> MRGSHHHHHHGSMVAPTSNPGVPDELDGVPAVVDCDVHAVLPSPHSLIPYLDEYWADQLVAQLAPTYEPNYHPRGSAIAQHSDASVDENGRAATTAENLVKDVFADGFTDFAVVNCLYGVQQIHQPRREMAHARALNHWIANEWLDKDDRLRASIVVPQGSPRAAAEEIDFWSGDKRFVQVLLLGQSELLYGREINWPIWEAAEAAGLPVTLHIGGVFRQAPTSVGWPASHLEWYVGQQSNIEAQLNSIISEGILQKFPKTKILLSELGFNWLPPFMWKFDKLWKSYRPDIPWVQESPLELIREHVRVTTSPSDGAEEAGRLDSIVDRLGSDRMLVYSSDYPHKHHSGPRDIENGTHSPELLDRIYRRNAFDLYNLVVPSPGKVG;> MTIIEHGSLGTLPAPSVTTGIVDADIHPVPQDGALEPYLDDRWKKHIREYGVRTTTGLQFISE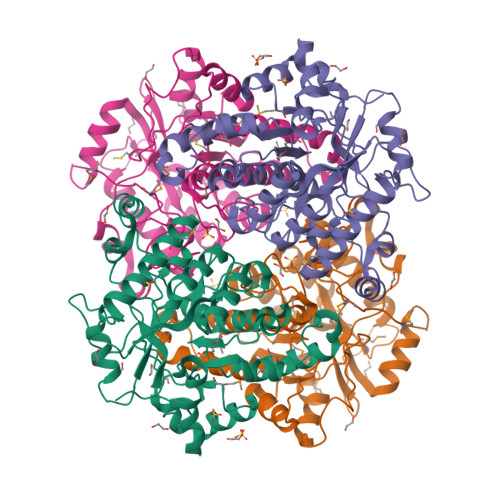YPQMYGGAMRADAWPESGYPGSDRELLRTQLLDKHNIQLGVLQCLAPGGQTLNPAGQALNQELAAALCRATNDWQLEHLVYPDPRMRAAIPVTFETPDYAVAEIERVGADPGVVAVLGTSKTLEPLGSRKYWPIYEASVAQNLPIQFHLSQGGGHANTGTGWTSYHTEYHTGHVQSFQSQLLSLVLSGTFDRFPTLKVMFVEGNVAHFAPLIQRMDYTWETLRGELPDLQRKPSEYIRDHIWASTQPIDEPEKPEHLAELLEEFCGDNVVFATDYPHFDFDDPETAFPRSFPVDLRDKILRGNGMRFFGVTNQAD> QEEE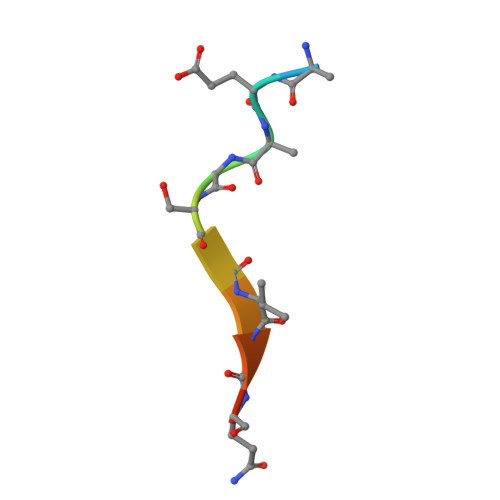GSGVGQGG> LLKALKK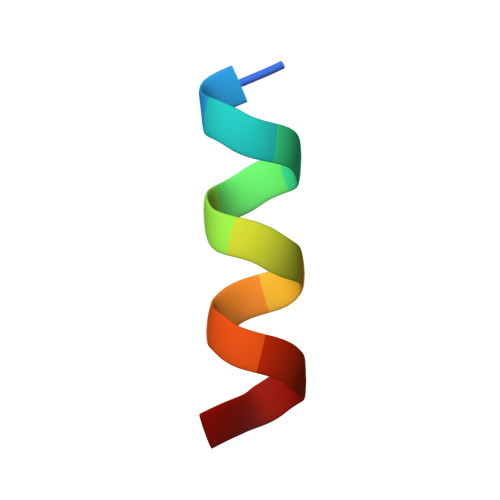LAKKYK> SLRNID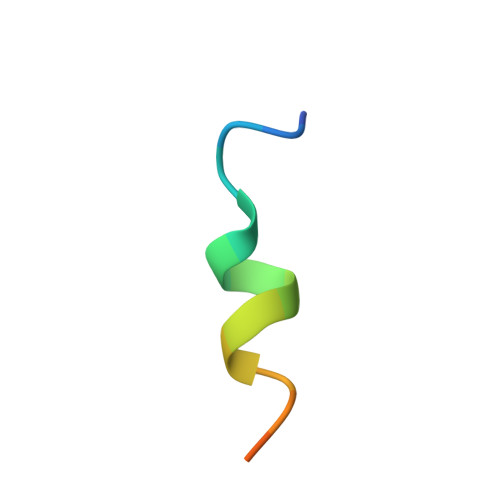DILDDIEGDLT(2R,3R,4S,5S,6R)-3,5-dihydroxy-4-{[(1E)-{3-hydroxy-2-methyl-5-[(phosphonooxy)methyl]pyridin-4-yl}methylidene]amino}-6-methyltetrahydro-2H-pyran-2-yl [(2R,3S,5R)-3-hydroxy-5-(5-methyl-2,4-dioxo-3,4-dihydropyrimidin-1(2H)-yl)tetrahydrofuran-2-yl]methyl dihydrogen diphosphate | C24 H35 N4 O19 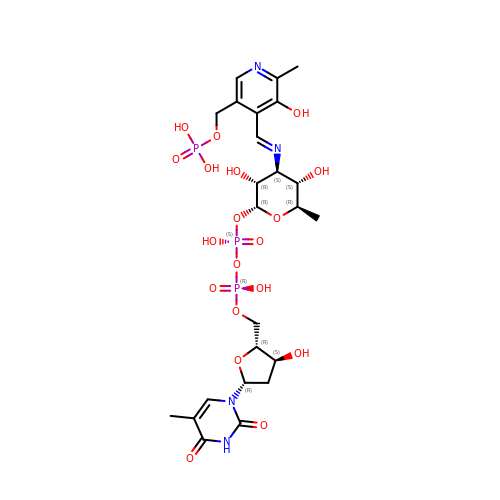P3 | UJDWKFAFGYHSFM-HMSDFHDVSA-N DIBROMOMETHANE | C H2 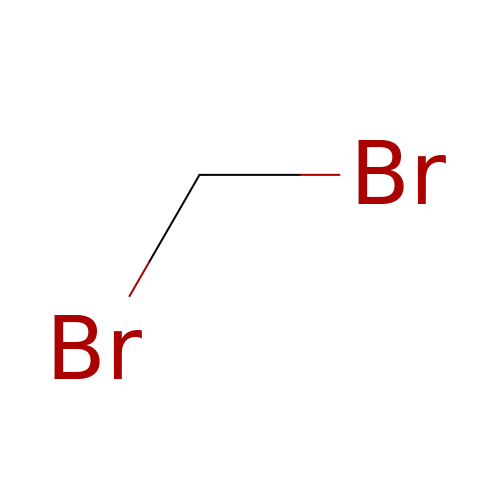Br2 | FJBFPHVGVWTDIP-UHFFFAOYSA-N> IIPVEEENPDFWNREAAEALGAAKKLQPAQTAAKNLIIFLGDGMGVSTVTAARILKGQKKDKLGPEIPLAMDRFPYVALSKTYNVDKHVPDSGATATAYLCGVKGNFQTIGLSAAARFNQCNTTRGNEVISVMNRAKKAGKSVGVVTTTRVQHASPAGTYAHTVNRNWYSDADVPASARQEGCQDIATQLISNMDIDVILGGGRKYMFRMGTPDPEYPDDYSQGGTRLDGKNLVQEWLAKRQGARYVWNRTELMQASLDPSVTHLMGLFEPGDMKYEIHRDSTLDPSLMEMTEAALRLLSRNPRGFFLFVEGGRIDHGHHESRAYRALTETIMFDDAIERAGQLTSEEDTLSLVTADHSHVFSFGGYPLRGSSIFGLAPGKARDRKAYTVLLYGNGPGYVLKDGARPDVTESESGSPEYRQQSAVPLDEETHAGEDVAVFARGPQAHLVHGVQEQTFIAHVMAFAACLEPYTACDLAPPAGTTDAAHPGRSVV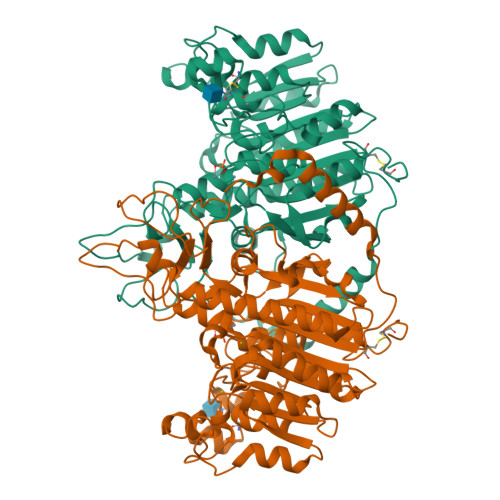PALLPLLAGTLLLLETATAP Microbial epoxide hydrolases, cis-epoxysuccinate hydrolases (CESHs), have been utilized for commercial production of enantiomerically pure L(+)- and D(−)-tartaric acids for decades. All these three CESH[L]s exhibit high sequence identity (>60%) with L-2-haloacid dehalogenases, which are members of the haloacid dehalogenase (HAD)-like superfamily. Studies have shown that both RhCESH[L] and KlCESH[L] adopt a two-step catalytic reaction mechanism by 18O-labeling studies.

We also constructed an inactive mutant, KlCESH[L]-D48N, to obtain the enzyme-substrate structure because D48 was proposed to be the first step catalytic residue. The first step was proposed to be a nucleophilic attack on the carbon atom in the oxirane ring by residue D18 in RhCESH[L] and residue D48 in KlCESH[L], forming an enzyme-substrate intermediate and opening the ring with an unidentified proton donor. However, the binding of non-catalytic ligands, including sulfate ions and products L-TA, did not cause significant structural changes.

>[4x]MGLKALFFNVQGTLVDFYSTITREGEAFSAVRGFQADWTTVTEQWRAEYRSRLDQVIKGERPWTTTDRIYREALDGILANHPWGASLNSADRDELNSLWSKLIPWDDTAPGLARLRSKYITSTLSNGSMASVLRISKLGALPFDAILTAELVRSSKPDPKVYQLALDSVGIEAHQAMMVACHKYDLQAAKRLGFKVAFIARPFEFGPNKKVDTKPEQYFDYYANSVVELAGMLGALEHHHHHH> QNVLVDDVNKLANGFNQLTASVSKLALTTSSALQAIQAVVNQNAAQVESLVSGITENFGAISTNFKVISQRLDKLE;> GKNLTADMSKLNISAEIQLINEIAHNVSNMRVEVEA

Virus entry of CoV is mediated by its spike (S) protein, where its S1 domain facilitates attachment to host cells, and its S2 domain is involved in the subsequent fusion between the virus and host membrane. During the fusion process, two heptad repeats, HR1 and HR2, in the S2 domain, assemble into a six-helix membrane fusion structure termed the fusion core. The formation of a six-helix bundle (6-HB) fusion core brings the virus closer to the cell membrane and promotes membrane fusion and infection. In this study, we have determined the fusion core structures of CCoV-HuPn-2018 and SADS-CoV at 2.10 Å and 2.59 Å, respectively, thus further completing the structural profiles of α-HCoVs fusion cores.

Here, we designed a linked recombinant SADS-CoV S2 fusion protein (HR1-HR2) using N-terminal residues 764–842 and C-terminal residues 1025–1061, with a six-amino-acid linker (L6: SGGRGG) between the two regions. The structure was refined to a final resolution of 2.59 Å with Rwork of 23.4% and Rfree of 28.2%. HR1 of SADS-CoV forms a 19-turn α-helix trimer, while these residues first form the random coil tether (residues 1025–1036) and then a second heptad repeat region (HR2) between residues 1037–1050, followed by the other extended conformation residues 1051–1061. HR1s from three HR1-L6-HR2 (SADS-CoV) molecules are arranged around the crystallographic three-fold symmetry axis and also form the central hydrophobic core in an antiparallel manner, resulting in a six-helical bundle structure with dimensions of ~107 Å in length and 30 Å in diameter with a left-handed supercoil. The HR2 helices make five full turns and pack into the central HR1 trimer to form a highly stable six-helix bundle conformation that coordinates the fusogenic events between the virus and host cell membranes. Such a structure is typical for the CoVs fusion core and represents the post-fusion state of the SADS-CoV spike protein. Intriguingly, owing to a lack of 14 aa insertions, SADS-CoV harbors 19 turns in HR1. Consequently, HR2 motif of SADS-CoV has only five turns in the helix region, the first reported exception in α-HCoV genus. A structural comparison between SADS-CoV and SARS-CoV-2 fusion cores revealed a high degree of overall structural similarity with a root mean squared deviation (RMSD) of approximate 0.814 Å for 71 Cα atoms of a piece of HR1 protomer. Only three-pair polar side-chain to side-chain interactions were detected between the helical region of HR2 and HR1 of SADS-CoV.>MKIATITGVTKSPELQVTKAIGALILSSDVALSALTTEKISIYIERGNGSNVILANKVLLKDFILASTYGTENTQSDADNAMIALCELADEGSIYLADKESIKITLEDLISDKRYDLHGIEEPQQTNNLFFFEQKSVASEEFNKKIDVQGFDLAIMTVDDSVSDLSYQYSNGQVVKYLPFELQTLSRDIDPIQAVLSDGKVVQGLTDRLTLPLVAVVGIEINKSQGSIINFVVRCLKTV[10x];> MNFIQYIDDSYAVKVKEINSSEGFYINGIQTPFFILSVFIGNKRVTGVEFNNYDSLPMLSVINDLGNIDLNVIPQNYFAT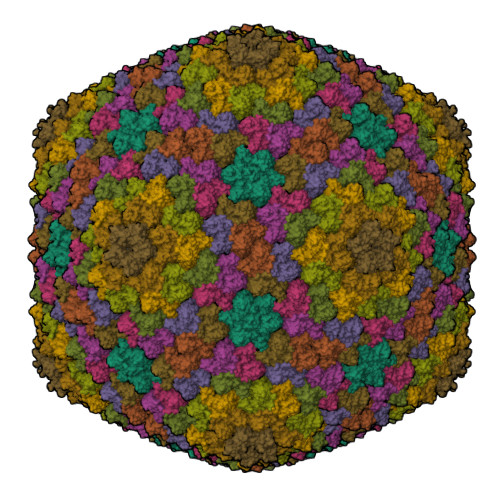AFTEIYFNIPF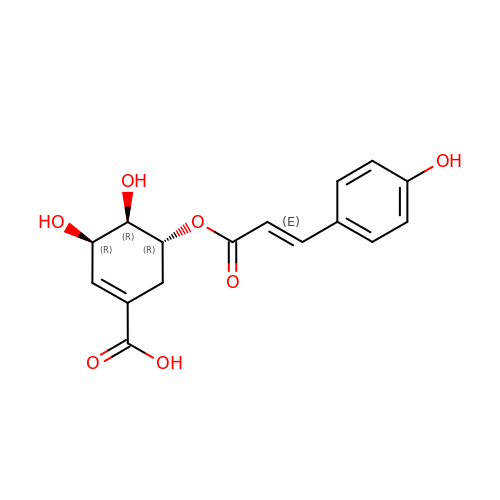(3~{R},4~{R},5~{R})-5-[(~{E})-3-(4-hydroxyphenyl)prop-2-enoyl]oxy-3,4-bis(oxidanyl)cyclohexene-1-carboxylic acid | C16 H16 O7 | GVECSFFLZYNEBO-PDXJTRCTSA-N>MGKYFGTDGVRGVANSELTPELAFKVGRFGGYVLTKDKQRPKVLIGRDTRISGHMLEGALVAGLLSIGAEVMRLGVISTPGVSYLTKAMDAEAGVMISASHNPVQDNGIKFFGGDGFKLSDEQEAEIERLMDEPEDKLPRPVGADLGLVNDYFEGGQKYLQFLKQTADEDFTGIHVALDCANGATSSLATHLFADLDADVSTMGTSPNGLNINDGVGSTHPEALSAFVKEKNADLGLAFDGDGDRLIAVDEKGNIVDGDQIMYICSKHLKSEGRLKDDTVVSTVMSNLGFYKALEKEGIKSVQTAVGDRYVVEAMKKDGYNVGGEQSGHLIFLDYNTTGDGLLSAIMLMNTLKATGKPLSELAAEMQKF[6x];>[6x]EAQQKTIEAITKAINYMAKRRIGALLTIERDTGMGDYIETGIPLNAKVSSELLINIFIPNTPLHDGAVIMKNNEIAAAACYLPLSESPFISKELG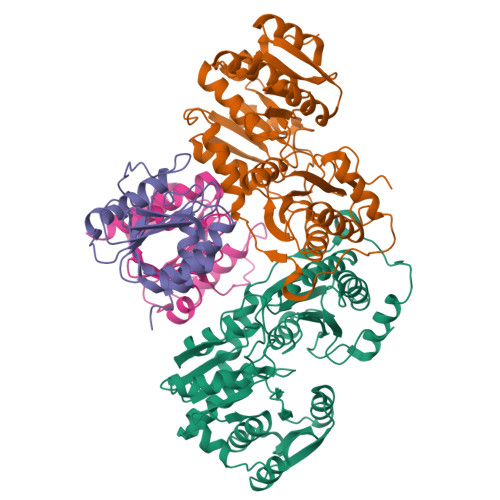TRHRAAVGISEVTDSLTIIVSEETGGVSVAKNGDLHRELTEEALKEMLEAEFKKNTRDTSSNRWYWRGKKNG>TPQNITDLCAEYHNTQIHTLNDKIFSYTESLAGKREMAIITFKNGATFQVEVPGSQAIDSQKKAIERMK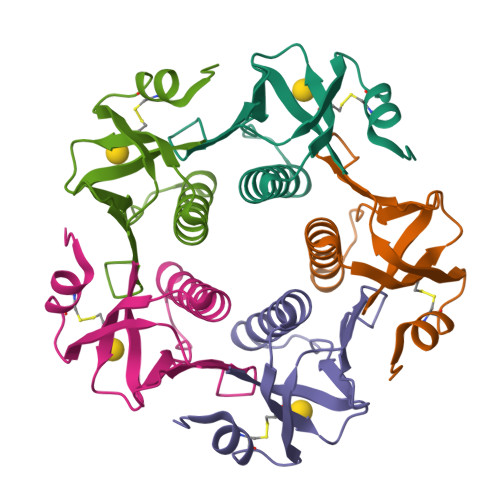DTLRIAYLTEAKVEKLCVWNNKTPHAIAAISMAN[5x]>[2x]VSDAVKKLRLPASMIIDGESPRFDDSIIPRHHGACFNVFIPAPPSHVPEVFTDRDITALIRAGGKDDELINKKISAKKIDHLHRQMLSFVTSRHNQAYWVSCRRETAAAGGLQTLGAFVEEQMTWAQTVVRHGGWFDEKDIDIILDTAIFVCNAFVTRFRLLHLSCVFDKQSELALIKQVAYLVAMGNRLVEACNLLGEVKLNFRGGLLLAFVLTIP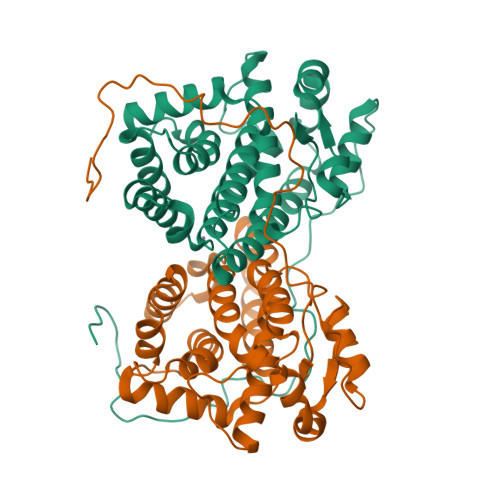GMQSRRSISARGQELFRTLLEYYRPGDVMGLLNVIVMEHHSLCRNSECAAATRAAMGSAKFNKGLFFYPLS> GPAWPEEKNYHQPAILNSSALRQIAEGTSISEMWQNDLQPLLIERYPGSPGSYAARQHIMQRIQRLQADWVLEIDTFLSQTPYGYRSFSNIISTLNPTAKRHLVLACHYDSKYFSHWNNRVFVGATDSAVPCAMMLELARALDKKLLSLKTVSDSKPDLSLQLIFFDGEEAFLHWSPQDSLYGSRH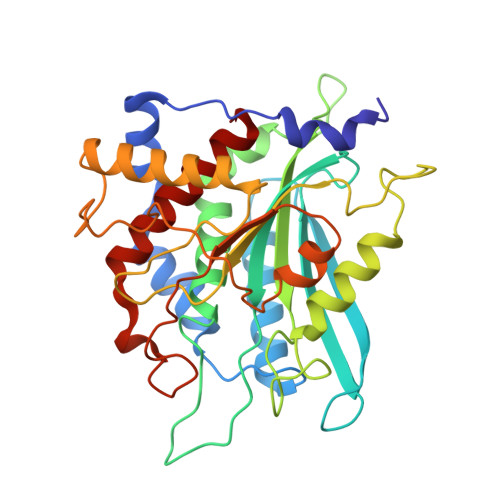LAAKMASTPHPPGARGTSQLHGMDLLVLLDLIGAPNPTFPNFFPNSARWFERLQAIEHELHELGLLKDHSLEGRYFQNYSYGGVIQDDHIPFLRRGVPVLHLIPSPFPEVWHTMDDNEENLDESTIDNLNKILQVFVLEYLHL>[4x]GSMTEIALIGNPNSGKTSLFNLITGHNQRVGNWPGVTVERKSGLVKKNKDLEIQDLPGIYSMSPYSPEAKVARD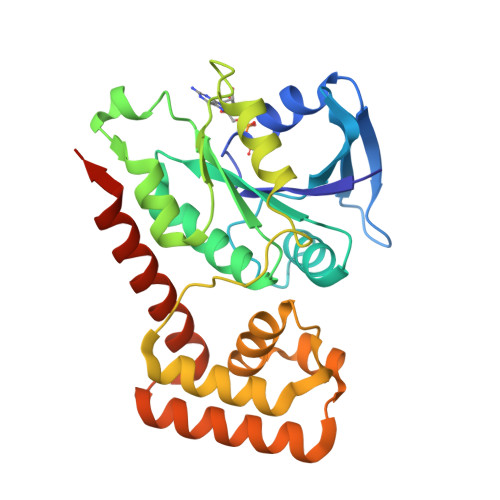YLLSQRADSILNVVDATNLERNLYLTTQLIETGIPVTIALNMIDVLDGQGKKINVDKLSYHLGVPVVATSALKQTGVDQVVKKAAHTTTSTVGDLAFPIYDDRLEAAISQILEVLGNSVPQRSARFYAIKLFEQDSLVEAELDLSQFQRKEIEDIIRITEEIFTEDAESIVINERYAFIERVCQMAESHTEDFALTLS> GSHMEVTEEDIAEIVSRWTGIPVSKLLEGEREKLLRLEEELHKRVVGQDEAIRAVADAIRRARAGLKDPNRPIGSFLFLGPTGVGKTELAKTLAATLFDTEEAMIQIDMTEYMEKHAVSRLIGAPPGYVGYEEGGQLTEAVRRRPYSVILFDEIEKAHPDVFNILLQILDDGRLTDSHGRTVDFRNTVIILTSNLGSPLILEGLQKGWPYERIRDEVFKVLQQHFRPEFLNRLDEIVVFRPLTKEQIRQIVEIQLSYLRARLAEKRISLELTEAAKDFLAERGYDPVFGARPLRRVIQRELETPLAQKILAGEVKEGDRVQVDVGPAGLVFAVPARVEA

The molecular chaperone ClpB, the bacterial homologue of Hsp104, is a disaggregation machine that provides thermotolerance by resolubilizing and reactivating aggregated proteins in concert with the DnaK (Hsp70) chaperone system. ClpB belongs to the family of AAA+ proteins (ATPases associated with various cellular activities) that comprises a wide range of molecular machines which utilize the energy from ATP hydrolysis to remodel their respective substrates. The AAA+ disaggregation machines Hsp104 and ClpB possess two NBDs per monomer, thus forming double-ring structures with 12 potential ATPase sites in the active hexameric complex. We determined high-resolution X-ray structures in different nucleotide states for one of the motor subunits, namely NBD2, of ClpB and combined the structural analysis with nucleotide-binding kinetics studies.

In addition to the AMPPCP-bound structure of ClpB NBD2 R621Q in the presence of MgCl2 and GdmCl, we also obtained the structure of this mutant variant in the ADP-bound state to a resolution of 2.1 Å. The mutant variant NBD2 R621Q is nucleotide-binding competent, but shows an approximately 30-fold reduced ATPase activity. Since the R621Q mutation selectively impairs ADP binding, we conclude that in the ADP state Arg621 contributes significantly to the nucleotide-binding energy, presumably by mimicking the nucleotide-associated Mg2+. In the ATP state, the Arg806 side chain must adopt an alternative conformation because otherwise it would clash with the γ-­phosphate. Indeed, Arg806 is located about 4 Å away from the nucleotide in the AMPPCP-bound structure. This is in agreement with our nucleotide-binding data, which show that the sensor 2 mutation R806A causes significantly impaired ADP binding but almost no change in ATP binding.> MAKSLPLNSRSKTTALKQPRELFSYARDIDGKYVYDDPENSLSYYYLPDSTIDTGIDLQGGYSKFKKIPDEQNLADFNSLLKAIIKYETSEGKKISSDIITFREIMTKILSLPYNLTDPIDLYVVPFDGQLFIKSDDELDMKRRKEQEVRMKQTNTVERYDYMKRCEYVGYKFETIATIPKPWSQVSRSQIENRNKKVVNNYEQYLSVIRTGIGNVKLVLAGEIDCCWDYLPDEQNKKLNHYVELKTSRIIENNSQVVSFEQKLFKAWCQCFLMGVTKIIYGFRDNNLILKNVELFNTEEIPILIKNNPLTNAATEKKINCTNALKWYGAVVDWLNTTVDKKDEIKSYRLKYDPVRKSFTLSETDSETNEKLRNGQL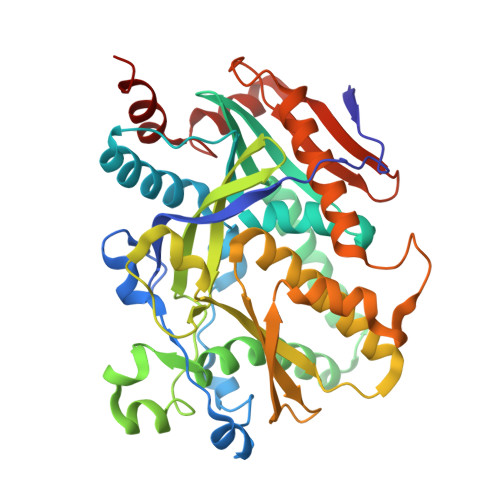LTPEFTEWRQSLKK>MDITQFSQLNPPSRLLMGPGPINADPRVLRAMSSQLIGQYDPAMTHYMNEVMALYRGVFRTENRWTMLVDGTSRAGIEAILVSAIRPGDKVLVPVFGRFGHLLCEIARRCRAEVHTIEVPWGEVFTPDQVEDAVKRIRPRLLLTVQGDTSTTMLQPLAELGEICRRYDALFYTDATASLGGNPLETDVWGLDAVSAGMQKCLGGPSGTSPITLSARMEEAIRRRKCVEEGIRTDAHRDGDEEMIYSNYFDLGMVMDYWGPERLNHHTEATTALFGARECA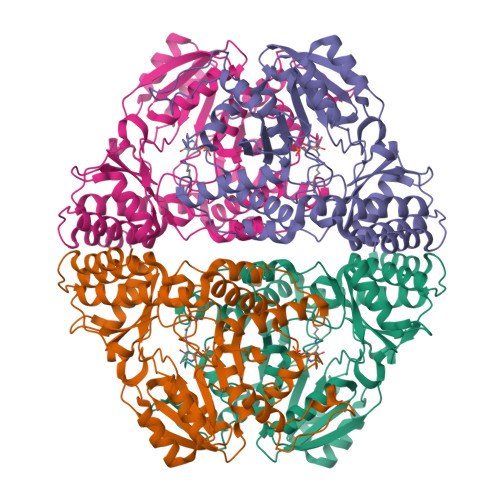RLILQEGLDYGIARHKLHGDALVKGIQAMGLETFGDLKHKMNNVLGVVIPQGINGDQARKLMLEDFGIEIGTSFGPLHGKVWRIGTMGYNARKDCVMTTLSALEAVLNYLKFPTTQGAAMQAAWDHYRSER[16x]> MGLVLTRKLKEAIQIGDDIEITVLAIQGD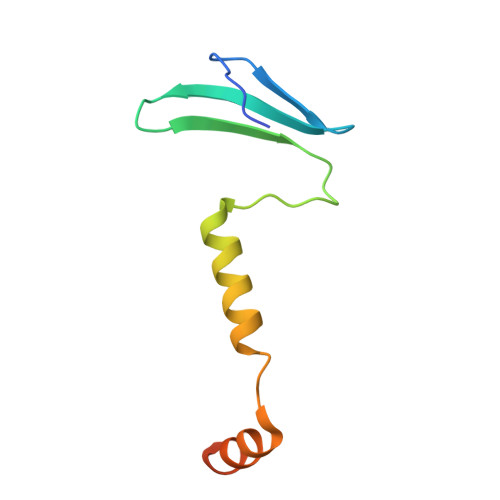QVKLGINAPKHVEIHRKEIYLAIQAENNAASHASKSSLKRLNEQLKHLKGGKQA> AQTVPYGIPLIKADKVQAQGFKGANVKVAVLDTGIQASHPDLNVVGGASFVAGEAYNTDGNGHGTHVAGTV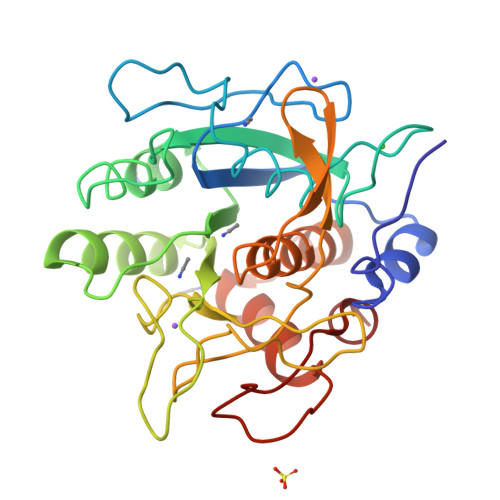AALDNTTGVLGVAPSVSLYAVKVLNSSGSGSYSGIVSGIEWATTNGMDVINMSLGGASGSTAMKQAVDNAYARGVVVVAAAGNSGNSGSTNTIGYPAKYDSVIAVGAVDSNSNRASFSSVGAELEVMAPGAGVYSTYPTNTYATLNGTSMASPHVAGAAALILSKHPNLSASQVRNRLSSTATYLGSSFYYGKGLINVEAAAQ>[3x]GSHMASKLKEAAEVTGSVSLEALEEVQVGENLEVGVGIDELV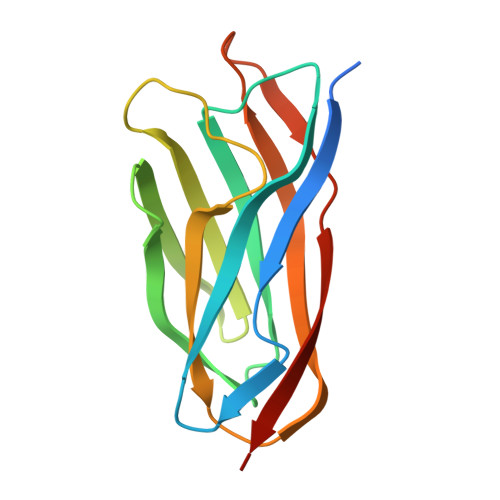NAEAFAYDFTLNYDENAFEYVEAISDDGVFVNAKKIEDGKVRVLVSSLTGEPLPAKEVLAKVVLRAEAKAEGSNLSVTNSSVGDGEGLVHEIAGTEKTVNIIEGTS> AMKPAQKGKTFSNVEIFDPPTNYRDPQVLYARPLELSDGTLLGTWENYSPEPPNVWFPIVKSKDGGKTWKEISKVKDTQNNWGLRYQPQLYELPRA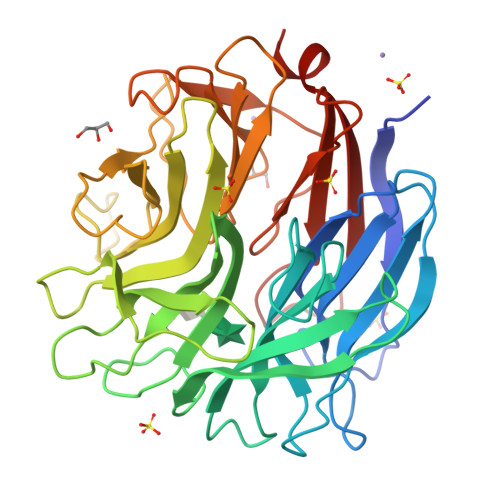FGKYPKGTVLCSGSSIPSDLSETLIEVYASRDKGYTWEFVSHVALGGEALPNPGLTPVWEPFLMTYKEKLILYYSDQRDNATHSQKLVHQTTTDLKKWSKVVDDTKYANYYARPGMPTVAKLPNNEYIYVYEYGGGPNPPAGSDYWFPVYYRLSKDPQKFLNKAHHQIVSNDGTTPAGSPYVVWTPYGGKNGTIVVSCGTRSEIFTNQALGDASAWKKWDVPQPTAYTRSLLTFQKDPDLLMIMGAGILPPAGGKNTVSASVVRLSEVMKS> MVGLTTLFWLGAIGMLVGTLAFAWAGRDAGSGERRYYVTLVGISGIAAVAYVVMALGVGWVPVAERTVFAPRYIDWILTTPLIVYFLGLLAGLDSREFGIVITLNTVVMLAGFAGAMVPGIERYALFGMGAVAFLGLVYYLVGPMTESASQRSSGIKSLYVRLRNLTVILWAIYPFIWLLGPPGVALLTPTVDVALIVYLDLVTKVGFGFIALDAAATLRAEHGESLAGVDTDAPAVADENSHHHHHHH

Bacteriorhodopsin (bR) from Halobacterium salinarum and sensory rhodopsin II from Natronomonas pharaonis (NpSRII) are intensively studied model systems which provide insight into how light is utilized for energy transduction or phototaxis, respectively. As with all microbial rhodopsins, both contain a buried retinal molecule that is covalently bound through a protonated Schiff base (SB) to a conserved lysine residue of helix G (Lys205 for NpSRII and Lys216 for bR). To understand how light-sensing in archaea is initiated by sensory rhodopsins, we perform serial synchrotron X-ray crystallography (SSX) studies of light induced conformational changes in sensory rhodopsin II (NpSRII) from the archaea Natronomonas pharaonis, both collecting time-resolved SSX data and collecting SSX data during continuous illumination.

X-ray diffraction data were then combined into sets corresponding to eight 30 ms time-windows, of which five (from 0 to 150 ms) were judged to have sufficiently high population of the photoactive state for further structural analysis. By representing difference Fourier electron density throughout a three-dimensional structure as a one-dimensional mapping onto the protein sequence, we observed that structural changes from 0 ms to 120 ms are highly-correlated and have internal Pearson correlation coefficients from 51% –71% and that this correlation drops to as low as 13% as the signal-to-noise falls on longer time-scale. The time-scale of this loss of correlation implies that photoactivated NpSRII microcrystals were swept out of the X-ray beam ~120 ms after photoactivation. By contrast, difference density features associated with helix G are weaker, yet are relatively constant until ∆t ≥ 120 ms, which is the time-scale when the photoactivated sample is swept from the X-ray beam position. In our SSX structure we modelled several n-Octyl-β-D-glucopyranoside (BOG) and Monoolein (MPG) molecules in similar positions to those previously observed.>[2x]KQEVQAWDGEVRQVSKHA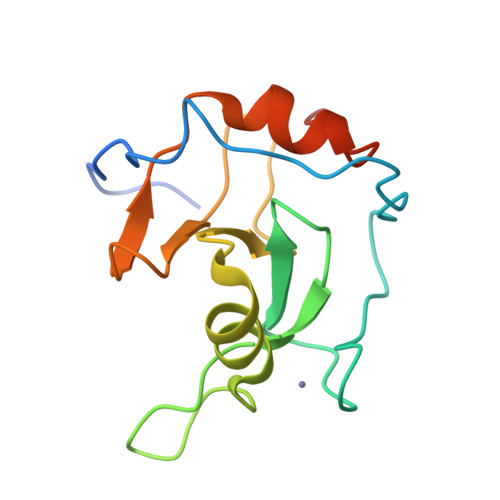FSLKQLDNPARIPPCGWKCSKCDMRENLWLNLTDGSILCGRRYFDGSGGNNHAVEHYRETGYPLAVKLGTITPDGADVYSYDEDDMVLDPSLAEHLSHFGIDMLKMQKTDK> MELAEKDKGRDFTLRNARMDDIDQIIKINRLTLPENYPYYFFVEHLKEYGLAFFVAIVDNSVVGYIMPRIEWGFSNIKQLPSLVRKGEVVSIAVLEEYRRKGIATTLLEASMKSMKNDYNAEEIYLHVRVSNYPAIALYEKLNFKKVKVLKGYYADGEDAYLMARPLHH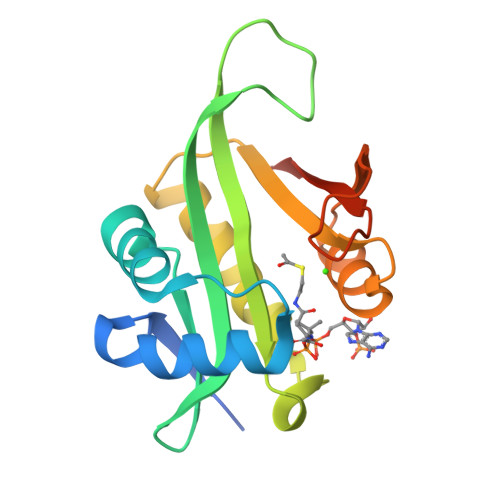HHHHPL>[2x]MSLKTGRSNIIAFIVPDQNPFFTEVLTEISHECQKHHLHVAVASSEENEDKQQDLIETFVSQNVSAIILVPVKSKFQMKREWLKIPIMTLDRELESTSLPSITVDNEEAAYIATKRVLESTCKEVGLLLANPNISTTIGRKNGY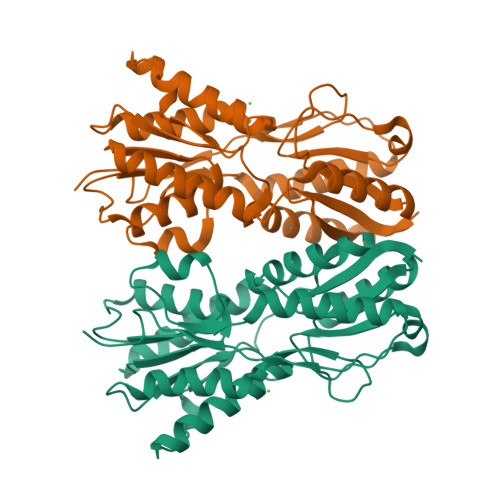NKAISEFDLNVNPSLIHYSDQQLGTNAQIYSGYEATKTLLSKGIKGIVATNHLLLLGALQAIKESEKEIKKDVIIVGFDDSYWNEIYTPKLTVISQPVKEMGQVAAKMIYKLIKGKDVTSIKLSTKLIIRESCSFNEGHHHHHH Here, we reveal a previously unannotated human DUB, OTULIN (also known as FAM105B), which is exquisitely specific for Met1 linkages. FAM105B comprises 352 amino acids (aa), and the OTU domain spans the majority of the protein (aa 80–352) and an N-terminal region with predicted helical content. Having established FAM105B as a Met1-linkage-specific OTU DUB, we named the enzyme OTULIN (OTU DUB with linear linkage specificity). Crystal structures of the OTULIN catalytic domain in complex with diubiquitin reveal Met1-specific Ub-binding sites and a mechanism of substrate-assisted catalysis in which the proximal Ub activates the catalytic triad of the protease.

Next, we determined the structure of OTULIN D336A to 1.35 Å resolution. There were no global structural perturbations, but His339 was now in the active rotamer, and Cys129 showed increased occupancy of the active rotamer. Consistently, Ub suicide inhibitors that did not modify wild-type (WT) OTULIN modified OTULIN D336A and also OTULIN N341D, in which the catalytic Asn341 was changed to a negatively charged Asp. Both mutants stabilize His339 in the active conformation, generating a more reactive enzyme. Next, we tested whether the more reactive OTULIN N341D or D336A mutants showed improved diUb hydrolysis activity. Strong effects of Glu16 mutation were also observed in the OTULIN D336A mutant.

> GPLSVAPEMDIMDYCKKEWRGNTQKATCMKMGYEEVSQKFTSIRRVRGDNYCALRATLFQAMSQAVGLPPWLQDPELMLLPEKLISKYNWIKQWKLGLKFDGKNEDLVDKIKESLTLLRKKWAGLAEMRTAEARQIACDELFTNEAEEYSLYEAVKFLMLNRAIELYNDKEKGKEVPFFSVLLFARDTSNDPGQLLRNHLNQVGHTGGLEQVEMFLLAYAVRHTIQVYRLSKYNTEEFITVYPTDPPKDWPVVTLIAEADRHYNIPVRVCEETSL>MTENFFGKTLAARPVEAIPGMLEFDIPVHGDNRGWFKENFQKEKMLPLGFPESFFAEGKLQNNVSFSRKNVLRGLHAEPWDKYISVADGGKVLGTWVDLREGETFGNTYQTVIDASKSIFVPRGVANGFQVLSDFVAYSYLVNDYWALELKPKYAFVNYADPSLDIKW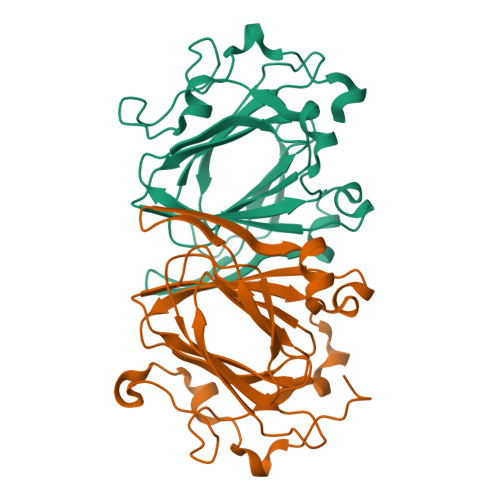ENLEEAEVSEADENHPFLKDVKPLRKEDL[2x]PDFs are ubiquitous essential metalloenzymes which co-translationally remove the formyl group carried by the initiator methionine in bacteria, mitochondria and chloroplast. Here, we present and characterize a PDF enzyme issued from the bacterium Streptococcus agalactiae (SaPDF) which behaves as an excellent structural platform to describe PDF-inhibitor interactions. Like most other PDFs, SaPDF behaves as a monomer and its crystal structure reveals a classical PDF fold. In addition, SaPDF contains the typical insertions of type 2 PDFs12, including an eight-amino acids loop folded as an α-helix (insertion 2) and a long loop connecting strands β2 and β3 usually referred as the CD-loop (insertion 3).

The ligand binding site is localized at the interface between the N and the C sub-domains, as evidenced by the structures of the complexes between SaPDF and synthetic tripeptides. Crystal-soaking experiments were conducted with formylated peptides (Fo-Met-Ala-Ser and Fo-Met-Ala-Arg) but led to deformylated molecules in the crystal structures as previously reported for other PDFs2627. This is due to the ability of the enzyme to deformylate formylated substrates in the crystal packing. Peptides, which therefore represent deformylation reaction products, were found bonded to SaPDF through a high number of non-covalent interactions, which are similar to those found previously with Escherichia coli PDF (EcPDF). Indeed, the free N-terminal amine group coordinated catalytic ion and was hydrogen bonded to the catalytic residue Glu175. The hydrophobic methionine side chain fitted into a deep hydrophobic S1’ pocket composed of several conserved residues (Val71, Leu125, Glu129, Tyr167, Val171, His174). Finally, peptides were in a conformation mimicking a β-strand which was hydrogen-bonded with the main backbone peptide bond of Gly130 from conserved motif II (E129GCLS133), Val71 from conserved motif I (G70VGLAAPQ77), and Gly69 which preceds motif I, linking the two β-sheets from N- and C-terminal sub-domains.

> MAAIDKLVKASHLIDMNDIIREGNPTLRKVAEEVTFPLSEKEEILGEKMMQFLKHSQDPIMAEKLGLRGGVGLAAPQLDISKRIIAVLVPNVEDAQGNPPKEAYSLQEVMYNPKVVSHSVQDAALSDGEGCLSVDREVPGYVVRHARVTIEYFDKTGEKHRLKLKGYNSIVVQHEIDHIDGIMFYDRINEKNPFAVKEGLLILE;> MAS> SMLKREDWYDLTRTTNWTPKYVTENELFPEEMSGARGISMEAWEKYDEPYKITYPEYVSIQREKDSGAYSIKAALERDGFVDRADPGWVSTMQLHFGAIALEEYAASTAEARMARFAKAPGNRNMATFGMMDENRHGQIQLYFPYANVKRSRKWDWAHKAIHTNEWAAIAARSFFDDMMMTRDSVAVSIM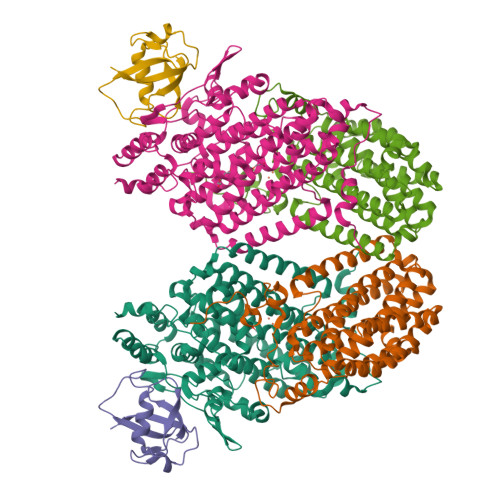LTFAFETGFTNMQFLGLAADAAEAGDHTFASLISSIQTDESRHAQQGGPSLKILVENGKKDEAQQMVDVAIWRSWKLFSVLTGPIMDYYTPLESRNQSFKEFMLEWIVAQFERQLLDLGLDKPWYWDQFMQDLDETHHGMHLGVWYWRPTVWWDPAAGVSPEEREWLEEKYPGWNDTWGQCWDVITDNLVNGKPELTVPETLPTICNMCNLPIAHTPGNKWNVKDYQLEYEGRLYHFGSEADRWCFQIDPERYKNHTNLVDRFLKGEIQPADLAGALMYMSLEPGVMGDDAHDYEWVKAYQ;> ALKPLKTWSHLAGNRRRPSEYEVVSTNLHYFTDNPERPWELDSNLPMQTWYKKYCFDSPLKHDDWNAFRDPDQLVYRTYNLLQDGQESYVQGLFDQLNDRGHDQMLTREWVETLARFYTPARYLFHALQMGSVYIHQIAPASTITNCATYETADHLRWLTHTAYRTRELANCYPDVGFGKRERDVWENDPAWQGFRELIEKALIAWDWGEAFTAINLVTKPAVEEALLQQLGSLAQSEGDTLLGLLAQAQKRDAERHRRWSSALVKMALEKEGNREVLQKWVAKWEPLADKAIEAYCSALPDGENAIVEAKSASRYVRQMMG;> TFPIMSNFERDFVIQLVPVDTEDTMDQVAEKCAYHSINRRVHPQPEKILRVRRHEDGTLFPRGMIVSDAGLRPTETLDIIFMD> GGUUAAAGCCUUAUGGUCGCUACCAUUGCACUCCGGUAGCGUUAAAAGGGAAGACGGGUGAGAAUCCCGCGC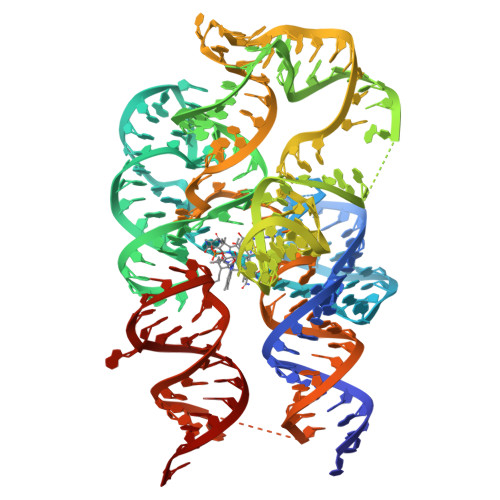AGCCCCCGCUACUGUGAGGGAGGACGAAGCCCUAGUAAGCCACUGCCGAAAGGUGGGAAGGCAGGGUGGAGGAUGAGUCCCGAGCCAGGAGACCUGCCAUAAGGUUUUAGAAGUUCGCCUUCGGGGGGAAGGUGAACA>[3x]ALTAKHRPSVVWLHNAECTGCTEAAIRTIKPYIDALILDTISLDYQETIMAAAGEAAEAALHQALEGKDGYYLVVEGGLPTIDGGQWGMVAGHPMIETTKKAAAKAKGIICIGTCSAYGGVQKAKPNPSQAKGVSEALGVKTINIPGCPPNPINFVGAVVHVLTKGIPDLDENGRPKLFYGELVHDNCPRLPHFEASEFAPSFDSEEAKKGFCLYELGCKGPVTYNNCPKVLFNQVNWPVQAGHPCLGCSEPDFWDTMTPFYEQG;>[3x]AESKPTPQSTFTGPIVVDPITRIEGHLRIMVEVENGKVKDAWSSSQLFRGLEIILKGRDPRDAQHFTQRACGVCTYVHALASSRCVDDAVKVSIPANARMMRNLVMASQYLHDHLVHFYHLHALDWVDVTAALKADPNKAAKLAASIAPARPGNSAKALKAVQDKLKAFVESGQLGIFTNAYFLGGHKAYYLPPEVDLI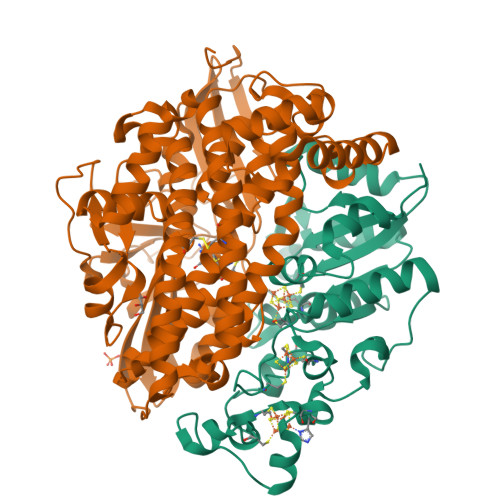ATAHYLEALHMQVKAASAMAILGGKNPHTQFTVVGGCSNYQGLTKDPLANYLALSKEVCQFVNECYIPDLLAVAGFYKDWGGIGGTSNYLAFGEFATDDSSPEKHLATSQFPSGVITGRDLGKVDNVDLGAIYEDVKYSWYAPGGDGKHPYDGVTDPKYTKLDDKDHYSWMKAPRYKGKAMEVGPLARTFIAYAKGQPDFKKVVDMVLGKLSVPATALHSTLGRTAARGIETAIVCANMEKWIKEMADSGAKDNTLCAKWEMPEESKGVGLADAPRGALSHWIRIKGKKIDNFQLVVPCTWNLGPRGAQGDKSPVEEALIGTPIADPKRPVEILRTVHAFDPCIACGVH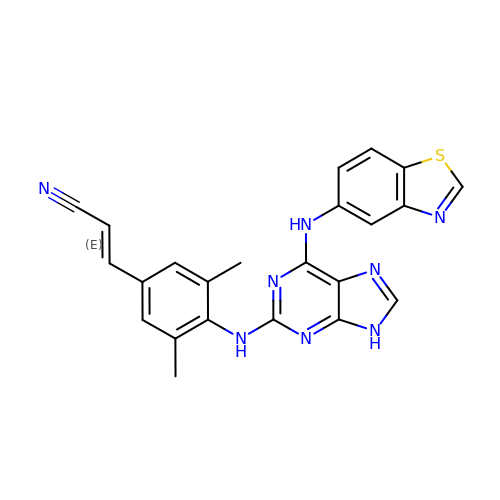(2E)-3-(4-{[6-(1,3-benzothiazol-5-ylamino)-9H-purin-2-yl]amino}-3,5-dimethylphenyl)prop-2-enenitrile | C23 H18 N8 S | FZDPEDQCVGYRLP-ONEGZZNKSA-N>[2x]SELSFNYPNFQSVEDITFQGGASPRNETLQLTPTDSNGIPIRQRAGHAVYSQPFQLRDTSFYTTFTFVIRTTSNSPADGFAIFIAPPDFPVKRYGGYLGLFEPNTATNTSANKVVAVEFDTWVNTEWKEPRYRHIGIDVNSIVSVRVTRWQDKDVFSRSIATAHVGYDGISKILTAFVTYPDGGNYVLSHVVDLAEIFPGDVRIGFSGATGQYETQYIHSWSFSSTSTNLLRDGARHHHHHH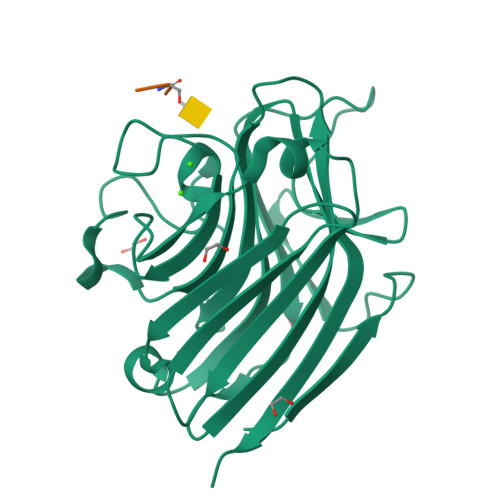;>[2x]XSSVG> AGCAT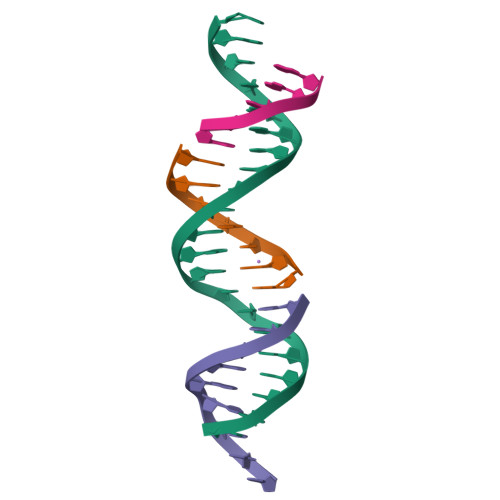GA;> CACTGACTCATGCTCATCTGA;> TGTCAGATG;> GTCAG Oligopeptidase B (OPB, EC 3.4.21.83), an enzyme belonging to the prolyl oligopeptidase (PREP) family, has recently emerged as a virulence factor in T. brucei and other trypanosomes, and is a potential therapeutic target. OPB hydrolyses peptide substrates of up to 30 amino acid residues in length, after arginine or lysine with a preference for arginine and most efficiently after a pair of basic residues. The overall structure of TbOPB comprises the typical 2 domain α/β-hydrolase and β-propeller architecture that is present in all members of the PREP family structurally characterized to date. A short N-terminal segment (residues 1–87) and long C-terminal segment (residues 436–714) together form the α/β-hydrolase domain, whilst the region in between (residues 88–435) forms the β-propeller domain.

TbOPB was cocrystallised with the inhibitor antipain to investigate the structural features responsible for substrate recognition, specificity and catalysis. Electron density was visible for all active site residues and the covalently bound antipain inhibitor. The catalytic triad Asp648, His683, and Ser563, form the charge relay and Ser563 has reacted with the P1 aldehyde of antipain to form a covalent hemiacetal transition state analogue complex. The oxyanion is stabilized by hydrogen bonding to the NH group of Ala564, the residue that follows the catalytic Ser in the sequence, as is characteristic of α/β-hydrolase enzymes. The oxyanion is further stabilized by hydrogen bonding to the OH group of Tyr482, as observed for LmOPB and the related PREP and DPP4, but not AAP that instead has another hydrogen bond to a main chain NH. The primary specificity for a P1 Arg is provided by specific interactions with Glu607 and Glu655. The main chain carbonyl of Arg650 also contacts the guanidinium group of the P1 Arg, and additional specificity is provided by a π-stacking interaction with the side chain of Phe589. The P2 carbonyl is hydrogen bonded to the important Arg650, and this interaction is also conserved in PREP and AAP. In LmOPB the P3 Arg interacts with Ser523 and Leu617, whilst in TbOPB an alternative conformer was adopted, resulting in interactions with Asp214 and Lys208 of the propeller domain. The TbOPB-antipain closed state structure aligned with the equivalent LmOPB structure with a root mean square deviation (RMSD) of 0.59 Å for 588 CA atoms.

>[6x]MQTERGPIAAHRPHEVVFGKVEGEDRGANPMDPPRRRVDPLFWLRDDNRADPEVLAHLHLEKDYYEKRAVDIKDLAETIYQEHISHIEETDMSAPYVYDRFLYYTRDVKGLSYKLHCRVPAGKTPGEGEDEEIVLDENKLAEGKSFCVVGCVAPAPPEHALVAYSVDYCGDEVYSIRFVRDVVADKVEGTNGSVVWGPNAECFFYITKDASKRDNKVWRHIIGQPQSEDVCLYTDDDPLFSVGVGRSGDGKTLIICSMSSETSESHLLDLRKGVKHNTLEMVRPREKGVRYTVEMHGTDTLIVLTNKDKCVNGKVVLTKRSAPTDWGTVLIPHDDKVTIDDVAVFAKFAVLSGRRDGLTRVWTVRLGPDNLFSSATLKELHFDEPVFTAHVVCSQMKTYDASLLRLRYSSMTTPTVWYDEDVLSGERKVVKARKVGGGFESKNYVCRRELATAPDGTKVPISLVYDTSIDLKKPNPTMLYGYGSYGICIEPEFNSRFLPYVDRGMIYAIAHVRGGGEMGRTWYEVGGKYLTKRNTFMDFIACAEHLISSGLTTPAQLSCEGRSAGGLLVGAVLNMRPDLFHVALAGVPFVDVMTTMCDPSIPLTTGEWEEWGNPNEYKFFDYMNSYSPIDNVRAQDYPHLMIQAGLHDPRVAYWEPAKWASKLRELKTDSNEVLLKMDLESGHFSASDRYKYLRENAIQQAFVLKHLNVRQLLRK;>[6x]FRVR>GSELFRGVLQVSSNVLDCANDNWWCSLLDLDTSDWEPLTHTNRLMAIYLSSVASKLDFTGGPLAGCLYFFQVECNKFEEGYHIHVVIGGPGLNPRNLTVCVEGLFNNVLYHLVTGNVKLKFLPGMTTKGKYFRDGEQFIENYLMKKIPLNVVWCVTNIDGYIDTCISATFRRGACHA[2x]

The nuclease domain of NS1 (NS1_Nuc) is responsible for DNA Ori binding and nicking that is critical for B19V viral DNA replication. NS1 contains one nuclease domain (Nuc, aa 1–176), one helicase domain (aa 302–457) and one transactivation domain (TAD, aa 523–531). NS1 belongs to the HUH-endonuclease superfamily and it shares conserved ssDNA cleavage mechanism with other HUH-endonuclease members. NS1_Nuc is of α/β fold in nature.

Totally, two NS1_Nuc structures (Form I and Form II) were solved. The Form II structure belongs to P21 space group. It was refined to 2.2-Å resolution with final Rwork and Rfree of 22.3 % and 25.8 %, respectively. Different from the Form I structure, there are two NS1_Nuc molecules within the asymmetric unit of the Form II structure. Superposition showed that the overall folding of NS1_Nuc is very similar in the two structures; the root mean square deviation (RMSD) value is 0.8 Å, based on 169 pairs of Cα atoms. The conformations of the α-helices and -strands are well conserved, but NS1_Nuc does show some conformational changes, especially in the βlinker and β4-β5 linker regions. Compared to the Form II structure, Glu77 is shifted about 7.3 Å in the Form I structure. As observed in the Form I and Form II NS1_Nuc structures, Leu121 can adopt two different conformations, but neither are compatible with A-5 in the WDV Rep/ssDNA complex structure. However, as supported by the clear 2Fo-Fc electron density maps, Arg94 is well defined and adopts similar conformations in our NS1_Nuc structures. The β4-α5linker contains two highly conserved Lys residues, Lys127 and Lys129. Different from Arg94, both Lys127 and Lys129 can undergo subtle conformational changes.>[4x]GHMYQHHNWQGALLDYPVSKVVCVGSNYAKHIKEMGSAVPEEPVLFIKPETALCDLRQPLAIPSDFGSVHHEVELAVL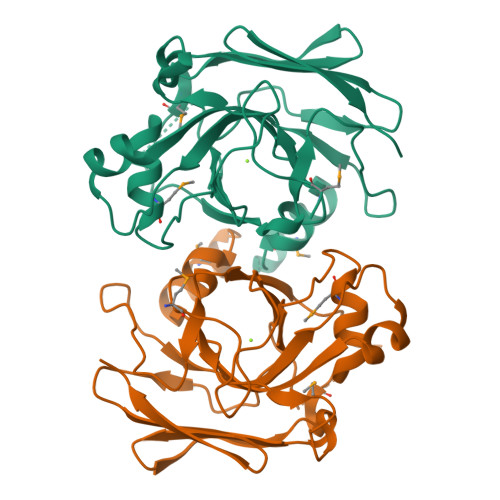IGATLRQATEEHVRKAIAGYGVALDLTLRDVQGKMKKAGQPWEKAKAFDNSCPLSGFIPAAEFTGDPQNTTLSLSVNGEQRQQGTTADMIHKIVPLIAYMSKFFTLKAGDVVLTGTPDGVGPLQSGDELTVTFDGHSLTTRVLGS> MDLIQAAYFVVAILFIVGLKRMAHPTTAKSGIVWAGWGMVLAVLATFFWPGMGNFALILLALLLGSVVAWWAAVRVAMTDMPQMVAIYNGMGGGAAATIAAVELLKGAFENTGLMALAILGGLIGSVAFTGSLIAFAKLQGIMKSRPILFPGQKAVNALVLALTVVIGLSLLWNDATASIVLFFLLALLFGVLMTLPIGGGDMPVAISFYNAFTGMAVGFEGFAVGNPALMVAGTLVGAAGTLLTVLMARAMNRSVWSVLVGGFGVEQEAGEVKGSLKPIDVEDAAVMLAYAGKVVFVPGYGMALSQAQHKLKELADLLEARGVEVKFAIHPVAGRMPGHMNVLLAEAGVDYDKLKDLEEINPEFPTVDVAVVIGANDVVNPAARRPGSPLYGM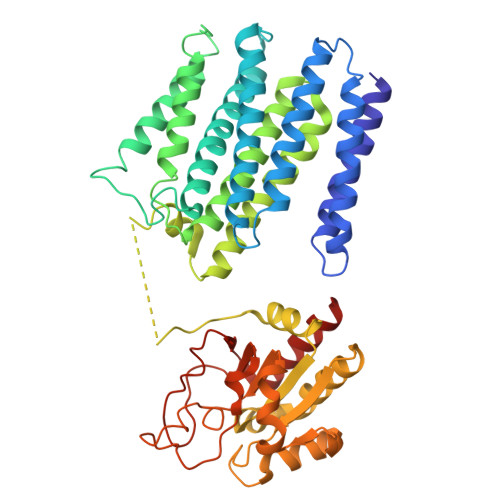PILDVDKAKNVIVIKRGQGKGFAGVENELFYAENTRMLYGDAQKVLTELIQALKRL We recently characterized two novel HSL family esterases from the thermophilic fungus Rhizomucor miehei: RmEstA and RmEstB. The physiological substrates of RmEstA and RmEstB detected in our studies have been found to be short-chain triacylglycerol, linalyl acetate, and butyl butyrate. Both of these enzymes belong to the α/β hydrolases and exhibit distinct substrate specificities: RmEstA shows highest activity toward longer-chain esters, whereas RmEstB favors hydrolysis of shorter-chain esters. The three-dimensional structures of two HSL esterases from R. miehei, RmEstA and RmEstB, were determined. Both of the esterases were composed of a core catalytic domain and a cap domain, exhibiting the typical α/β-hydrolase fold. A classical catalytic triad consisting of Ser161 (Ser164 in RmEstB) as the nucleophile, His292 (His291 in RmEstB) as the proton acceptor/donor, and Asp262 (Asp261 in RmEstB) as the residue stabilizing the His was identified in RmEstA (RmEstB).

The crystal structures of RmEstA and RmEstB were determined at 2.41 Å and 2.27 Å resolutions, respectively. The triclinic space group of RmEstA was P1 with two monomers in the asymmetric unit. Amino acid residues 1–3 of RmEstA and the uncleaved C-terminal His-tag were not visible on the electron-density map. In the asymmetric unit, RmEstA formed a dimer in complex with three sulfates, and two of the sulfates interacted with two monomers via Arg104. Note that the third single sulfate was found in the crevice of two monomers, with four Arg residues from two monomers forming an arched area. The side chains of His292 and Asp262 in RmEstA were stabilized by a network of hydrogen bonds located at the carboxyl edge of β-strands 7 and 8, respectively. The substrate-binding pocket of RmEstA was a channel running through the whole protein and the entrance to this channel was surrounded by five α-helices (α1, α2, α6, α8, and α9), the 310-helix G2 (His197–Lys199) and the loop regions (His87–Gly90 and Ile291–Ala298). On the other hand, the substrate-binding pocket of RmEstA is a curved tunnel which can accommodate ester substrates with long acyl chains. RmEstA can hydrolyze esters of longer carbon chain lengths (up to C16), with the highest activity observed for C6 (15), whereas RmEstB favors the hydrolysis of esters with shorter carbon chain lengths, with highest activity observed for C2 (16). A structural comparison of RmEstA and RmEstB suggested that the differences in the substrate-binding pocket might make a marked contribution to their distinct substrate specificities.

>[2x]MTVGNPPIHPVYAAAFAAMKERPPIHTLDLKVVRESSEARQLAANIKLPEVIEEDKVVESDGKTLKLTIVRPPGTEDQILPVLIFLHGGGFVFGSKYTHIKPVRDLTVKANVVTVFVDYSLSPEAKFPTAIEEIYAAILWVRENASSLNINAEALAVAGDSAGATLSAAVSIYAKEKGLSAAIKTQVLIYPATAVSHAKYESYKLFGNGDYILSAEDLKFFSNAYLPAPASELNDKLATLELATKADLEGLPPALLFTAESDVLRDEGEKYAQQLAEAGVDVAAVRVLGAVHGFITVPVETPQYRFTINTIVAHLRDIYAKYNALEHHHHHH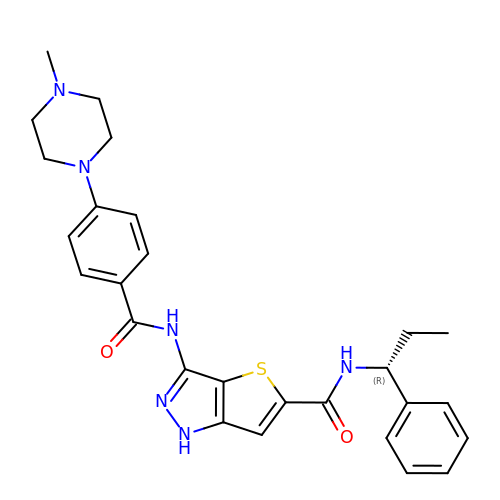3-({[4-(4-METHYLPIPERAZIN-1-YL)PHENYL]CARBONYL}AMINO)-N-[(1R)-1-PHENYLPROPYL]-1H-THIENO[3,2-C]PYRAZOLE-5-CARBOXAMIDE | C27 H30 N6 O2 S | BGKRQXRINOKEMF-OAQYLSRUSA-N(4S)-19-acetyl-4-[(1R)-1-hydroxy-2-({1-[3-(propan-2-yl)phenyl]cyclopropyl}amino)ethyl]-11-oxa-3,16-diazatricyclo[15.3.1.1~6,10~]docosa-1(21),6(22),7,9,17,19-hexaen-2-one | C35 H43 N3 O4 | 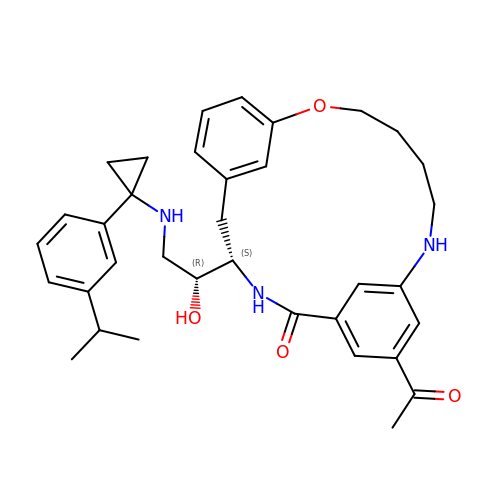LUJWXMKDHHFLOK-JHOUSYSJSA-N> MNNTDLIHLIKHFMHNELKAVEEVIDSPLSEFANLI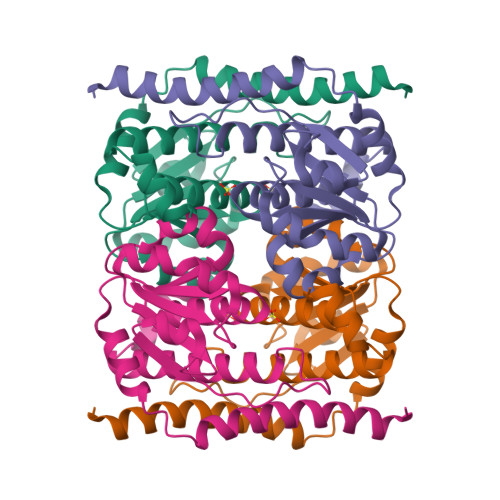KVLQSCQGKVVFIGVGKSGIIARKLAATFASTGTPSFFVHGTEAVHGDLGMVAKDDVVILISNSGETAEILATLPSLKKMGNYLISFTRSHHSSLAISCDLSVEIPVKSEADNLGLAPSCSSTVVLVVGDAVALALSELKKFTRADFGLYHPGGALGIKANS> GPLGSGETVKIVRIEKARDIPLGATVRNEMDSVIISRIVKGGAAEKSGLLHEGDEVLEINGIEIRGKD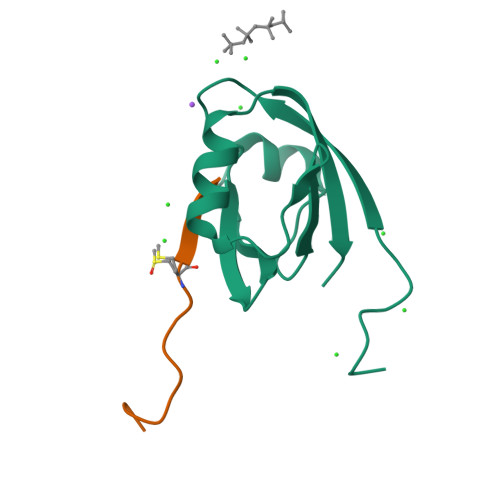VNEVFDLLSDMHGTLTFVLIPS;> RVEMWNLMPPPAMERLI> MACRCTQLQDTIDEVATQFYSSIHYLSSHHDFVPLPGQEKVSDSKVNPISAEELQFAQRDLAKDLVTKFM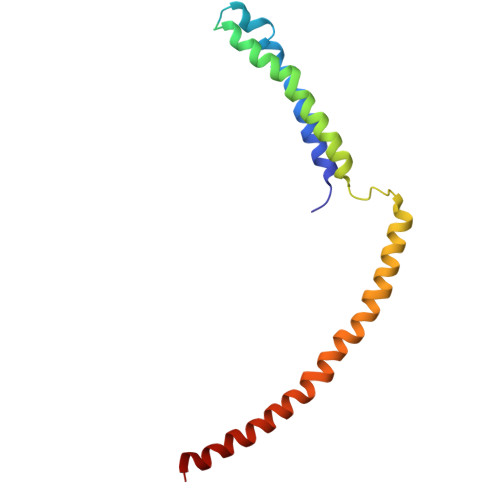QIDTLINQLPGISTAPKHQLEKIKKLQNSIEEKQLERKSLESENEDLKLQLAKRIETFGRLSCVLFQP>[2x]GDDNEIEIPKAPVLEKAQLALAIKSEEGAVTKTGETTPTDADVNTLTVGVFGVDGWSVIYTKDATPNSDGTKDVGPQEVYAGEAHVVVVANAAPVIQTELAKAKDITDFIETTINLSDETLTKGLTMSSKVLDVTLVANTTNYIGYDDEVGDITVKDISGKEVYGAGPVPLVRDVASIALAGADIGNPENANYESKSFVLKEVFIASAK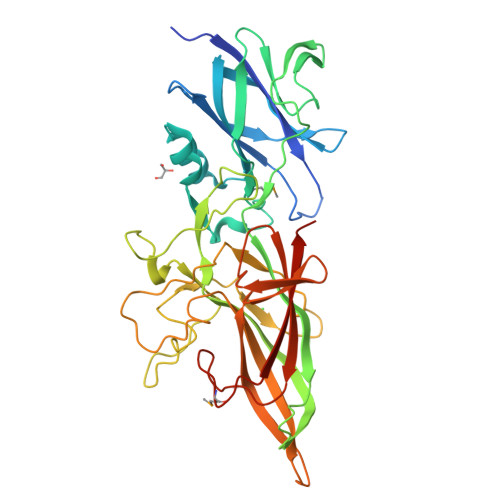GVSSVASTEEWGTIEKDFFGDTHFGYLDYKVGLLFLTSPNNIDEGSYKKGLQTKYDALAKKHVENDPALNHEFYVYENTKGEVKSGESNVNEAYANHTLLIVKGDYTYLPQGAKESITKENCYYAIPVGEEVTIDGTEKRSKFYVQRNYKYEISLTIIGPGSEIPYDPMISTNVSASVKVEPWNVKTIHEEVE>[2x]MNPTIIRARAPLRLGLAGGGTDVAPYADTFGGYVLNATIDRYAYAVIKTLTIPAVRFVSTDQQVEKHQLISEPLELNGTLNLHKAVYNHMIRNYNHGKPIALELSTFCDAPAGSGLGSSSTLVVVMIKAFVELLNLPLDDYAIAQLAYRIERVDCGLAGGRQDQYSATFGGFNFMEFYAAARTIVNPLRIKNWVLCELEASLVLFYTGVSRESAKIIQDQSDNVVSHKTAAIEAMHGIKREALVMKEALL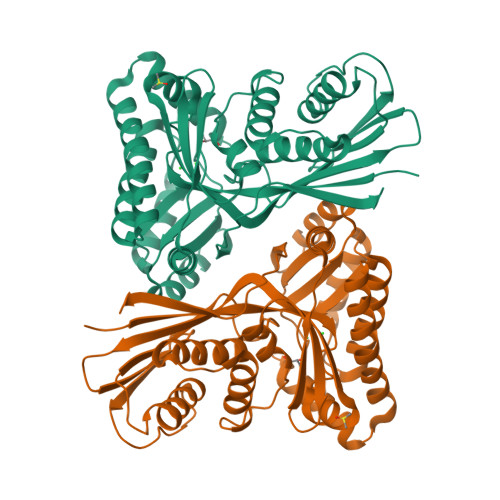KGDFKAFVASMRLGWDNKKNSARTVSNAHIDEIYDAAIRAGAQAGKVSGAGGGGFMLFFVPTEKRMDLIRTLGEYDGQVSNCHFTKNGTQAWRIAN4-METHYL-5-HYDROXYETHYLTHIAZOLE PHOSPHATE | C6 H10 N O4 P S | 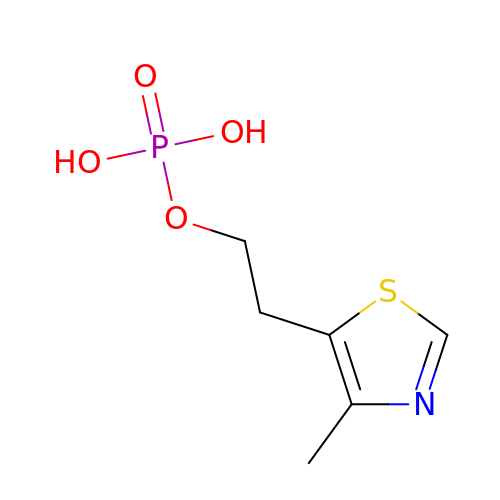OCYMERZCMYJQQO-UHFFFAOYSA-N> MGHHHHHHMMRSHYCGQLNESLDGQEVTLCGWVHRRRDHGGVIFLDVRDREGLAQVVFDPDRAETFAKADRVRSEFVVKITGKVRLRPEGARNPNMASGSIEVLGYELEVLNQAETPPFPLDEYSDVGEETRLRYRFIDLRRPEMAAKLKLRARITSSIRRYLDDNGFLDVETPILGRPTPEGARDYLVPSRTYPGHFFALPQSPQLFKQ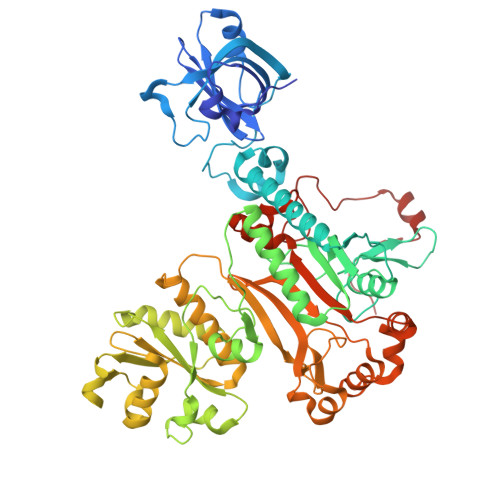LLMVAGFDRYYQIAKCFRDEDLRADRQPEFTQIDIETSFLDESDIIGITEKMVRQLFKEVLDVEFDEFPHMPFEEAMRRYGSDKPDLRIPLELVDVADQLKEVEFKVFSGPANDPKGRVAALRVPGAASMPRSQIDDYTKFVGIYGAKGLAYIKVNERAKGVEGLQSPIVKFIPEANLNVILDRVGAVDGDIVFFGADKAKIVCDALGALRIKVGHDLKLLTREWAPMWVVDFPMFEENDDGSLSALHHPFTSPKCTPAELEANPGAALSRAYDMVLNGTELGGGSIRIHDKSMQQAVFRVLGIDEAEQEEKFGFLLDALKYGAPPHGGLAFGLDRLVMLMTGASSIREVIAFPKTQSAGDVMTQAPGSVDGKALRELHIRLREQPKAE By hydrolyzing SAH to adenosine (Ado) and L-homocysteine (Hcy), the enzyme SAHase (SAH hydrolase) serves as an important regulator of SAM-dependent methylation through the control of the SAM:SAH ratio, and is an indicator of the biological methylation activity of the cell. SAHases are usually active as homotetramers. The protomer has a three-domain fold, with two prominent domains, the substrate- and cofactor-binding domains, separated by a deep crevice. A small C-terminal dimerization domain locks two subunits into a homodimer by quaternary complementation of the cofactor binding site, where a tightly but non-covalently bound nicotinamide adenine dinucleotide (NAD+) is found in its oxidized form.

The Zn2+ cation was incorporated into recombinant PaSAHase during expression and co-purifies with the enzyme. Co-purification of Zn2+ with PaSAHase indicates that the enzyme has a very high affinity for this cation. Specifically, our kinetics studies based on PaSAHase inactivation revealed that a tightly bound Zn2+ cation acts as a very strong noncompetitive inhibitor with an inhibitory constant Ki as low as 15 nM. Furthermore, the enzymatic study indicated that Zn2+ locks the enzyme-ligand complex in the closed conformation. Our crystal structures help to elucidate this puzzling behavior by showing that there is a tetrahedral zinc binding site, formed by three highly conserved amino acid residues involving S (Cys85), N (His323), and two O (Asp139) ligand atoms, located in the active site, where - together with the H323-F324 molecular gate - the divalent cation shuts access to the active site of the enzyme. Moreover, the Zn2+ cation is located at the interface between the two principal domains and is coordinated by three ligands from the substrate-binding domain (C85 Sγ, D139 O and D139 Oδ1) and one ligand from the cofactor-binding domain (H323 Nε1), thus further stabilizing the SAHaseclosed-Ligand-K+ complex. On the other hand, the potent inhibitory effect of Zn2+ is based on binding at the molecular gate and arresting the enzyme in the closed conformation.

>[4x]SNAMSAVMTPAGFTDYKVADITLAAWGRRELIIAESEMPALMGLRRKYAGQQPLKGAKILGCIHMTIQTGVLIETLVALGAEVRWSSCNIFSTQDQAAAAIAAAGIPVFAWKGETEEEYEWCIEQTILKDGQPWDANMVLDDGGDLTEILHKKYPQMLERIHGITEETTTGVHRLLDMLKNGTLKVPAINVNDSVTKSKNDNKYGCRHSLNDAIKRGTDHLLSGKQALVIGYGDVGKGSSQSLRQEGMIVKVAEVDPICAMQACMDGFEVVSPYKNGINDGTEASIDAALLGKIDLIVTTTGNVNVCDANMLKALKKRAVVCNIGHFDNEIDTAFMRKNWAWEEVKPQVHKIHRTGKDGFDAHNDDYLILLAEGRLVNLGNATGHPSRIMDGSFANQVLAQIHLFEQKYADLPAAEKAKRLSVEVLPKKLDEEVALEMVKGFGGVVTQLTPKQAEYIGVSVEGPFKPDTYRY> YRPISQGVSDLVGLPNQICLQKTTSTILKPRLISYTLPINTREGVCITDPLLAVDNGFFAYSHLEKIGSCTRGIAKQRIIGVGEVLDRGDKVPSMFMTNVWTPPNPSTIHHCSSTYHEDFYYTLCAVSHVGDPILNSTSWTESLSLIRLAVRPKSDSGDYNQKYIAITKVERGKYDKVMPYGPSGIKQGDTLYFPAVGFLPRTEFQYNDSNCPIIHCK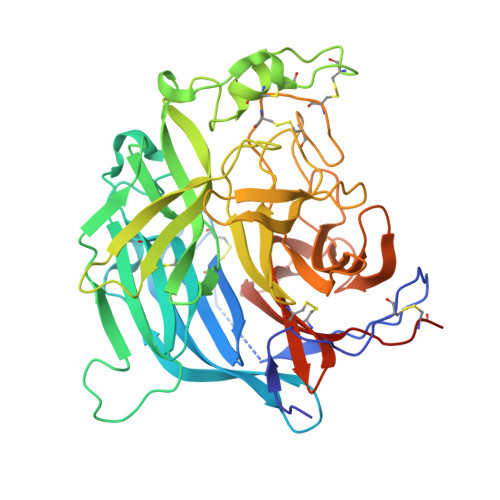YSKAENCRLSMGVNSKSHYILRSGLLKYNLSLGGDIILQFIEIADNRLTIGSPSKIYNSLGQPVFYQASYSWDTMIKLGDVDTVDPLRVQWRNNSVISRPGQSQCPRFNVCPEVCWEGTYNDAFLIDRLNWVSAGVYLNSNQTAENPVFAVFKDNEILYQVPLAEDDTNAQKTITDCFLLENVIWCISLVEIYDTGDSVIRPKLFAVKIPAQCSESGRGLVPR>MSHYKSNVRDQVFNLFEVFGVDKVLGADKFSDLDADTAREMLTEIARLAEGPIAESFVEGDRNPPVFDPETHTVTLPEGFKKSMRALFDGGWDKVGLAEHLGGIPMPRALQWALIEHILGANPAAYMYAGGPGMSEIFYNNGTDEQKKWATIAAERGWGATMVLTEPDAGSDVGAGRTKAVQQPDGTWHIEGVKRFITSADSDDLFENIMHLVLARPEGAGPGTKGLSLFFVPKFHFDHETGEIGERNGVFVTNVEHKMGLKVSATCELSLGQHGIPAVGWLVGEVHNGIAQMFDVIEQARMMVGTKAIATLSTGYLNALEYAKERVQGADMTQMTDKTAPRVTITHHPDVRRSLMTQKAYAEGLRAIYLYTATFQDAEVAQAVHGVDGDLAARVNDLLLPIVKGFGSETAYAKLTESLQTLGGSGFLQDYPIEQYIRDSKIDSLYAGTTAIQAQDFFFRKIIR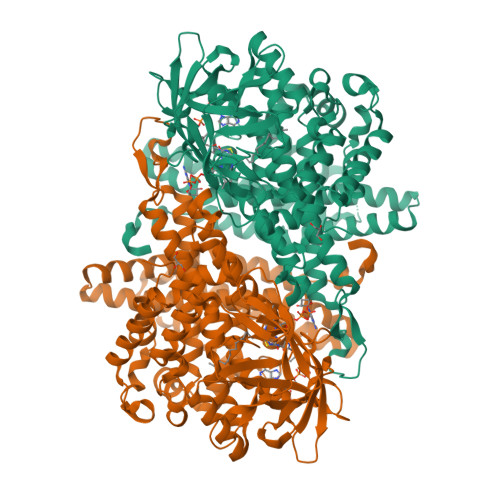DKGQALAYVAGEIEQFIKNENGNGRLKTERELLATALADVQGMAASLTGYLMAAQEDAASIYKVGLGSVRFLMAVGDLLSGWLLARQAAVAIEKLDAGATGADKSFYEGKIAAASFFAKNMLPLLTSTRQIIENLDNDVMELDEAAF[2x]> SGETSVPPGSALVGPSCVMDDFRDPQRWKECAKQGKMPCYFDLIEENVYLTERKKNKSHRDIKRMQCEC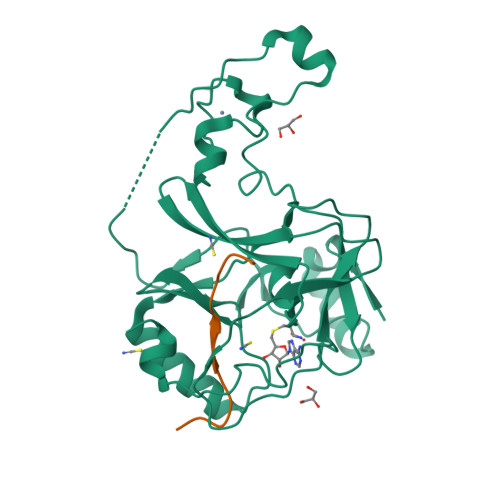TPLSKDERAQGEIACGEDCLNRLLMIECSSRCPNGDYCSNRRFQRKQHADVEVILTEKKGWGLRAAKDLPSNTFVLEYCGEVLDHKEFKARVKEYARNKNIHYYFMALKNDEIIDATQKGNCSRFMNHSCEPNCETQKWTVNGQLRVGFFTTKLVPSGSELTFDYQFQRYGKEAQKCFCGSANCRGYLGGENRVSIRAAGGKMKKERSRK;> APSTGGVIKPHRYR>MGAAILPDLGTEILIPVCAVIGIAFALFQWLLVSKVKLSAVRDASPNAAAKNGYNDYLIEEEEGINDHNVVVKCAEIQNAISEGATSFLFTEYKYVGIFMVAFAILIFLFLGSVEGFSTSPQACSYDKTKTCKPALATAIFSTVSFLLGGVTSLVSGFLGMKIATYANARTTLEARKGVGKAFITAFRSGAVMGFLLAANGLLVLYIAINLFKIYYGDDWGGLFSAITGYGLGGSSMALFGRVGGGIYTKAADVGADLVGKVERNIPEDDPRNPAVIADNVGDNVGDIAGMGSDLFGSYAESSCAALVVASISSFGLNHELTAMLYPLIVSSVGILVCLLTTLFATDFFEIKAVKEIEPALKKQLVISTVLMTIGVAVVSFVALPTSFTIFNFGVQKDVKSWQLFLCVAVGLWAGLIIGFVTEYYTSNAYSPVQDVADSCRTGAATNVIFGLALGYKSVIIPIFAIAISIFVSFTFAAMYGIAVAALGMLSTIATGLAIDAYGPISDNAGGIAEMAGMSHRIRERTDALDAAGNTTAAIG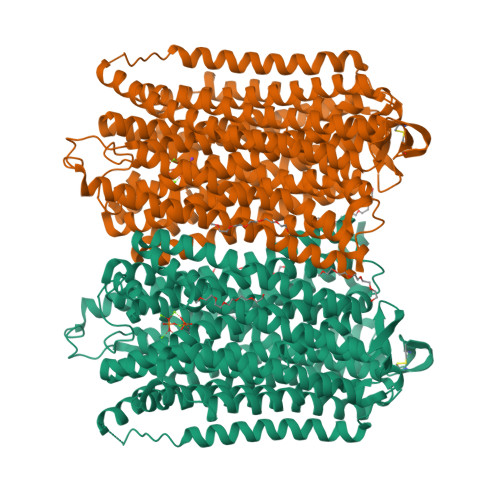KGFAIGSAALVSLALFGAFVSRASITTVDVLTPKVFIGLIVGAMLPYWFSAMTMKSVGSAALKMVEEVRRQFNTIPGLMEGTAKPDYATCVKISTDASIKEMIPPGALVMLTPLVVGILFGVETLSGVLAGSLVSGVQIAISASNTGGAWDNAKKYIEAGASEHARSLGPKGSDCHKAAVIGDTIGDPLKDTSGPSLNILIKLMAVESLVFAPFFATHGGLLFKIF[2x]> MPAHSFRIAAIPGDGIGLEVLPEGIRVLEAAALKHGLALEFDTFEWASCDYYLQHGKMMPDDWAEQLKQYDAIYFGAVGWPDKVPDHISLWGSLLKFRREFDQYVNIRPVRLFPGVPCALANRKVGDIDFVVVRENTEGEYSSLGGIMFENTENEIVIQESIFTRRGVDRILKYAFDLAEKRERKHVTSATKSNGMAISMPYWDKRTEAMAAHYPHVSWDKQHIDILCARFVLQPERFDVVVASNLFGDILSDLGPACAGTIGIAPSANLNPERNFPSLFEPVHGSAPDIFGKNIANPIAMIWSGALMLEFLGQGDERYQRAHDDMLNAIERVI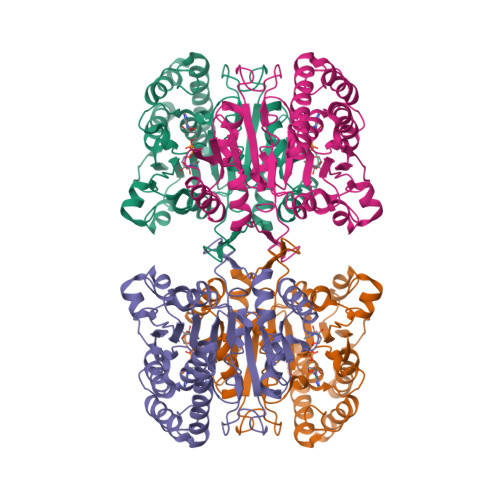ADGSVTPDMGGTLSTQQVGAAISDTLARLD>GSSGSSGSLEVSVGKATTIYAINGSSILLPCTFSSCYGFENLYFKWSYNNSETSRILIDGIVKNDKSDPKVRVKDDDRITLEGSTKEKTNNISILLSDLEFSDTGRYTCFVRNPKEKDLNNSATIFLQVVDKLEKVDN[2x]

Voltage-gated sodium channels are transmembrane proteins responsible for the generation of action potentials, and play important roles in the modulation of electrical impulses. They consist of a pore-forming α subunit and one or more auxiliary β subunits. Each β subunit has an extracellular immunoglobulin (Ig) domain, a transmembrane domain, and an intracellular domain, except for the secreted form of β1B2. Furthermore, the β subunits function as cell adhesion molecules (CAMs).

We determined the structure of the mouse β4 subunit extracellular domain fragment (β4ex) by X-ray crystallography. Unlike the human β4 subunit extracellular domain fragment used in the previous crystallographic study, which had either the C58A or C131W mutation, the present fragment contains all three of the Cys residues. The molecular structure of β4ex is highly superimposable on that of the C58A mutant14, except for the N-terminal region and the mutated residues. The N-terminal region of β4 does not participate in the β-sheet of the Ig fold, and appears to be flexible. The β4ex structure exhibits a remarkable feature: a highly ordered multimeric assembly of β4ex molecules is formed in the crystal lattice, and the β4ex molecules interact with each other in an antiparallel manner. The antiparallel arrangement is mediated by the interaction of the C″–D loop of one β4 molecule with strands B, D, and E of the β-sheet composed of strands B, E–E′, and D–D′ of the other β4 molecule. The side chain of Arg94 in the C″–D loop hydrogen bonds with the side and main chains of Ser48 in strand B. The side chain of Asp97 in the C″–D loop hydrogen bonds with the side chain of Asn113 in strand E. Val95, in the C″–D loop, participates in a hydrophobic interaction with Leu50 in strand B. This antiparallel interface is asymmetric between the two β4ex molecules, and can successively array the β4ex molecules in a linear manner. In the present β4 structure, this disulfide bond is not formed at a distance of 3.3 Å. The antiparallel arrangement is unambiguously related to the interface for the trans homophilic interaction of β4 in cell-cell adhesion, based on structure-based mutagenesis and site-directed photo-crosslinking.methyl 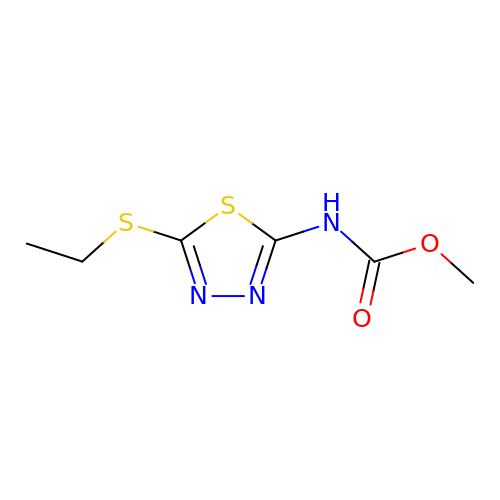~{N}-(5-ethylsulfanyl-1,3,4-thiadiazol-2-yl)carbamate | C6 H9 N3 O2 S2 | SSCYIPXZAWJONZ-UHFFFAOYSA-N2-{2-[2-(2-{4-[(alpha-D-mannopyranosyloxy)methyl]-1H-1,2,3-triazol-1-yl}ethoxy)ethoxy]ethoxy}ethyl 2-[3,6-bis(diethylamino)-9H-xanthen-9-yl]benzoate | C45 H61 N5 O12 | 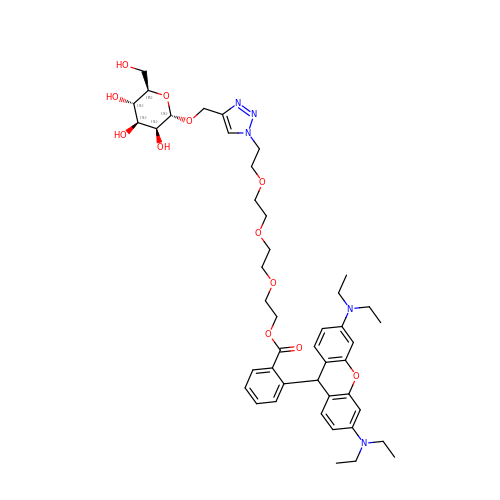NMXJNHVQXYBXDU-ZOLSBRMLSA-N> RHKILHRLL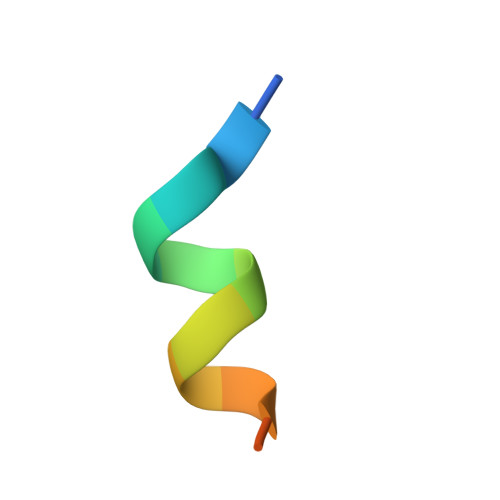QEGS>GAINKNMKLGQKVLIPVKQFPKFNFVGKLLGPRGNSLKRLQEETLTKMSILGKGSMRDKAKEEELRKSGEAKYFHLNDDLHVLIEVFAPPAEAYARMGHALEEIKKFLIPDYNDEIRQAQLQELTYLN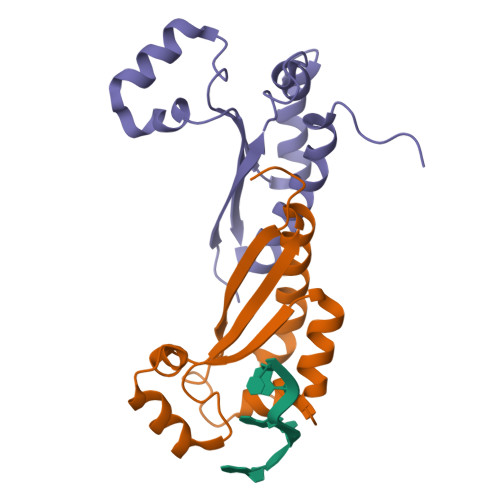GGSENADV[2x]> YQQDQVVKEDNIEAVGKKLHKYNTQFQEKSREYDRLYEEYTRTSQEIQMKRTAIEAFNETIKIFEEQCQTQERYSKEYIEKFKREGNEKEIQRIMHNYDKLKSRISEIIDS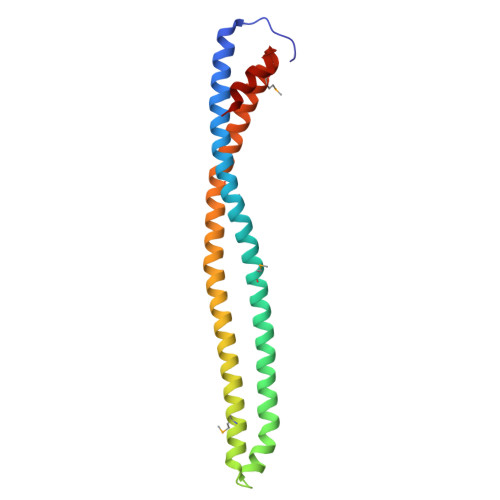RRRLEEDLKKQAAEYREIDKRMNSIKPDLIQLRKTRDQYLMWLTQKGVRQKKLNEWLGN>[4x]MYYIAIDIGGTQIKSAVIDKQLNMFDYQQISTPDNKSELITDKVYEIVTGYMKQYQLIQPVIGISSAGVVDEQKGEIVYAGPTIPNYKGTNFKRLLKSLSPYVKVKNDVNAALLG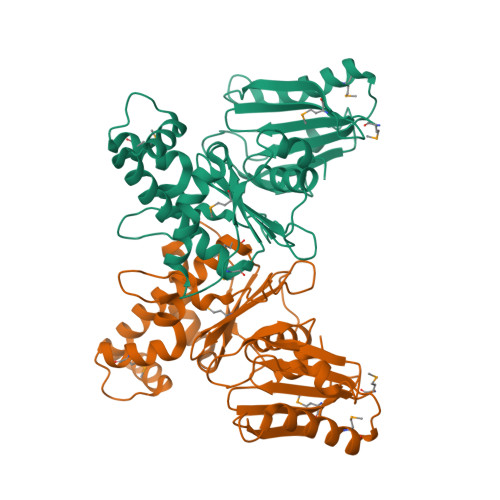ELKLHQYQAERIFCMTLGTGIGGAYKNNQGHIDNGELHKANEVGYLLYRPTENTTFEQRAATSALKKRMIAGGFTRSTHVPVLFEAAEEGDDIAKQILNEWAEDVAEGIAQIQVMYDPGLILIGGGISEQGDNLIKYIEPKVAHYLPKDYVYAPIQTTKSKNDAALYGCLQ>SRLNRESVIDAALELLNETGIDGLTTRKLAQKLGIEQPTLYWHVKNKRALLDALAVEILARHHDYSLPAAGESWQSFLRNAAMSFRRALLRYRDGAKVHLGTRPDEKQYDTVETQLRFMTENGFSLRDGLYAISA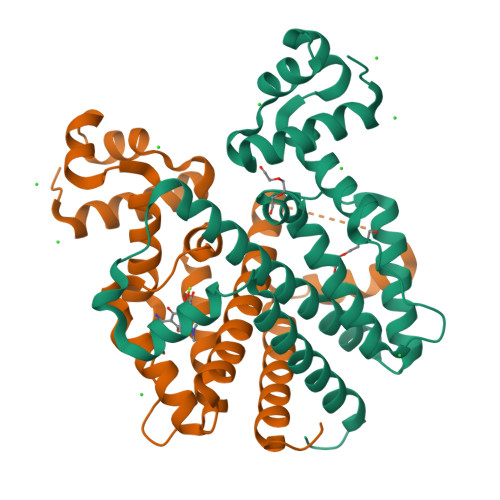VSHFTLGAVLEQQEHTAALTDRPAAPDENLPPLLREALQIMDSDDGEQAFLHGLESLIRGFEVQLTALLQIV[2x]> MKKGHHHHHHLVPRGSRKKIFKPEELRQALMPTLEALYRQDPESLPFRQPVDPQLLGIPDYFDIVKNPMDLSTIKRKLDTGQYQ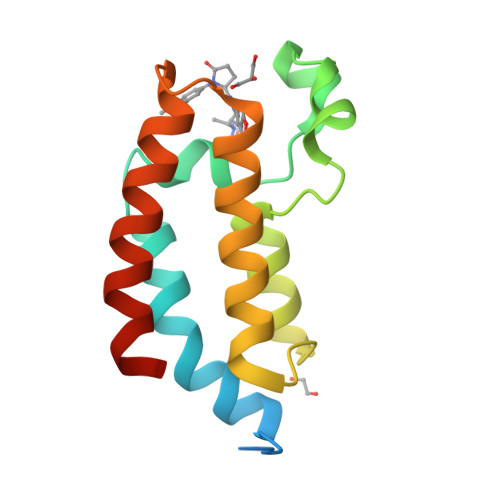EPWQYVDDVWLMFNNAWLYNRKTSRVYKFCSKLAEVFEQEIDPVMQSLG>[8x]MTESPERGRKRLGIYLAHFLDH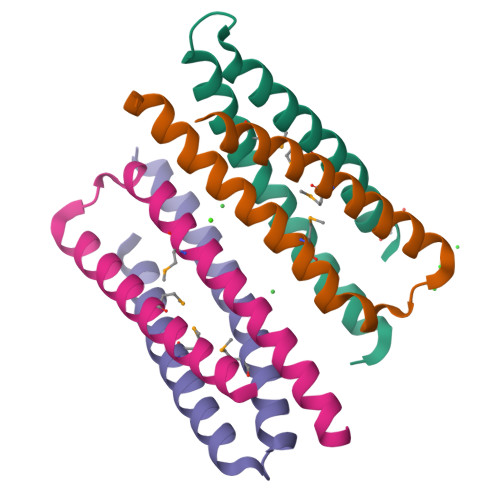VEGHMGEIGVQRDALAEDARLGALIDRALADMAVARASLNAVLRDL N-(3,5-dichlorobenzene-1-carbonyl)-5,5-dimethyl-L-norleucine 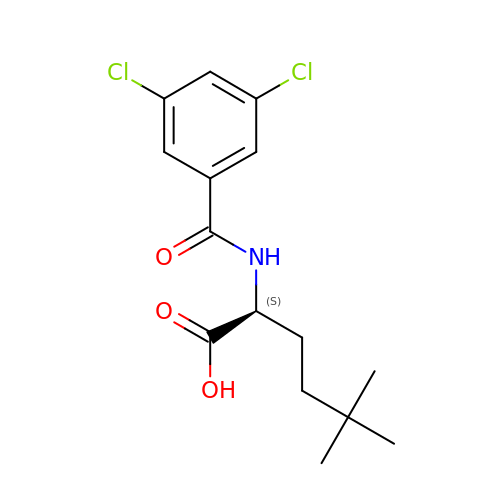| C15 H19 Cl2 N O3 | GTMNLKRWZVHZAV-LBPRGKRZSA-N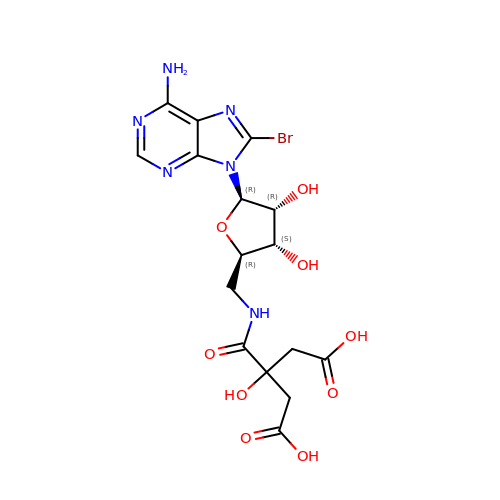8-bromo-5'-{[3-carboxy-2-(carboxymethyl)-2-hydroxypropanoyl]amino}-5'-deoxyadenosine | C16 H19 Br N6 O9 | QQTQAKWRRPPHOE-MSTPSEHLSA-N> SS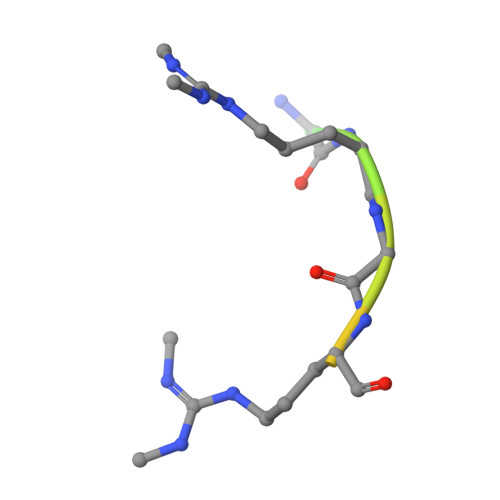GPARGRGRHPGKGVK>[2x]MAILAARIAVSNLHKETKKVFSDVMEDLYNYINPHNGKHSPMVAKSTLDIVLANKDRLNSAIIYDRDFSYNYFGFKTLERSYLLKINGKVAERPQHMLMRVSVGIHKEDIDAAIETYNLLSERWFTHASPTLFNAGTNRPQLSSCFLLSMKDDSIEGIYDTLKQC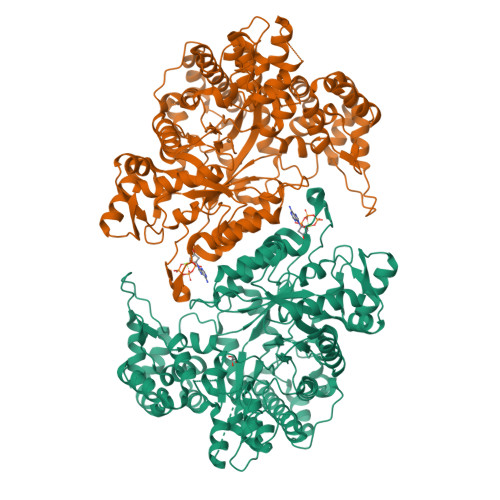ALISKSAGGIGVAVSCIRATGSYIAGTNGNSNGLVPMLRVYNNTARYVDQGGNKRPGAFAIYLEPWHLDIFEFLDLKKNTGKEEQRARDLFFALWIPDLFMKRVETNQDWSLMCPNECPGLDEVWGEEFEKLYASYEKQGRVRKVVKAQQLWYAIIESQTETGTPYMLYKDSCNRKSNQQNLGTIKCSNLCTEIVEYTSKDEVAVCNLASLALNMYVTSEHTYDFKKLAEVTKVVVRNLNKIIDINYYPVPEACLSNKRHRPIGIGVQGLADAFILMRYPFESAEAQLLNKQIFETIYYGALEASCDLAKEQGPYETYEGSPVSKGILQYDMWNVTPTDLWDWKVLKEKIAKYGIRNSLLIAPMPTASTAQILGNNESIEPYTSNIYTRRVLSGEFQIVNPHLLKDLTERGLWHEEMKNQIIACNGSIQSIPEIPDDLKQLYKTVWEISQKTVLKMAAERGAFIDQSQSLNIHIAEPNYGKLTSMHFYGWKQGLKTGMYYLRTRAHHHHHH Ca2+-regulated photoproteins are members of the EF-hand Ca2+-binding protein superfamily that provide bright flash-type bioluminescence to a great number of marine cnidarians and ctenophores. Photoproteins consist of a single polypeptide chain with a molecular weight of around 22 kDa to which the oxygenated CTZ, 2-hydroperoxycoelenterazine (2-hydroperoxyCTZ), is tightly but non-covalently bound. Photoprotein bioluminescence is greatly accelerated by binding of calcium ions to the EF-hand Ca2+-binding sites of a protein. CTZ-v has the same effect on photoprotein bioluminescence spectra; obelin activated with CTZ-v (obelin-v) demonstrates red-shifted bioluminescence with a peak at 532 and a shoulder at 415 nm while obelin with native CTZ emits light with a maximum at 480 nm and a shoulder at 400 nm.

Here, we report the crystal structure of semi-synthetic Ca2+-discharged obelin-v bound with the reaction product determined at 2.1 Å resolution. The final model includes two protein chains (A, B) with 192 and 191 of the 195 amino acid residues, correspondingly, two coelenteramine-v (CTM-v) molecules, six DMSO molecules, and 341 solvent molecules. Due to the crystallization conditions Ca2+-discharged obelin-v structure does not contain bound Ca2+ ions, because citrate is a calcium chelator. However, in the first Ca2+-binding loop of Ca2+-discharged obelin-v in both protein chains A and B (residues 29–37) there is an electron density which plausibly corresponds to Na+. Ca2+-discharged conformation of obelin-v is a globular molecule with the radius of ~ 25 Å, formed by the two sets of four helices designated as A–D and E–H in the N- and C-terminal domains, respectively. CTM-v resides in hydrophobic internal cavity of Ca2+-discharged obelin in the same position but in different orientation compared to 2-hydroperoxyCTZ-v of obelin-v. CTM-v is rotated 180 degrees, so that 2-benzyl group of CTM-v is directed towards different set of amino acid residues compared to the corresponding 8-benzyl group of 2-hydroperoxyCTZ-v. Despite the ligand rotation, the OH group of CTM-v forms a hydrogen bond with His22, which is the bond commonly observed in other photoprotein structures. The second hydrogen bond formed by CTM-v directly with the adjacent amino acid residues is the bond between Tyr138 and amino group of CTM-v. However, Ca2+-discharged obelin-v also has a possible solvent-access opening located between Phe28, Leu29 of helix A, Ile42, Ala46, Ile50 of helix B, and Ser142 of helix F.

>MSSKYAVKLKTDFDNPRWIKRHKHMFDFLDINGNGKITLDEIVSKASDDICAKLEATPEQTKRHQVCVEAFFRGCGMEYGKEIAFPQFLDGWKQLATSELKKWARNEPTLIREWGDAVFDIFDKDGSGTITLDEWKAYGKISGISPSQEDCEATFRHCDLDNSGDLDVDEMTRQHLGFWYTLDPEADGLYGNGVP[2x]> QGPLGSSEQLKHCNGILKELLSKKHAAYAWPFY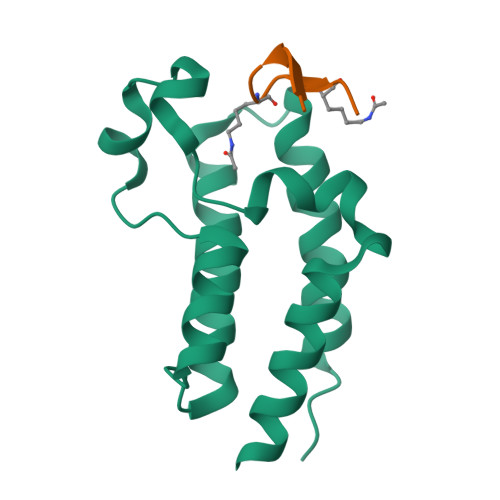KPVDASALGLHDYHDIIKHPMDLSTVKRKMENRDYRDAQEFAADVRLMFSNCYKYNPPDHDVVAMARKLQDVFEFRYAKMPD;> XWWIIPKVKKGCX> MQNEKLDHESVTQAMQPKDTPELRALYKSFEEESIIPLWTQLGDLMPIHPKSKAVPHVWKWSTLLRLARKSGELVPVGRGGERRALGLANPGLGGNAYISPTMWAAIQYLGPRETAPEHRHSQNAFRFVVEGEGVWTVVNGDPVRMSRGDLLLTPGWCFHGHMNDTDQPMAWIDGLDIPFSQQMDVGFFEFGSDRVTDYATPNFSRGERLWCHPGLRPLSGLQNTVASPIGAYRWEFTDRALTEQLLLEDEGQPATVAPGHAAIRYVNPTTGGDVMPTLRCEFHRLRAGTETATRNEVGSTVFQVFEGAGAVV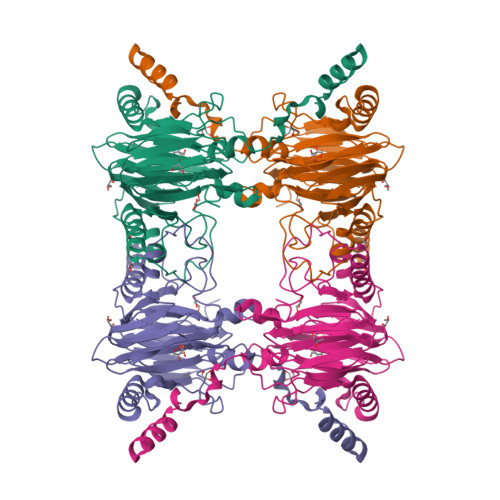MNGETTKLEKGDMFVVPSWVPWSLQAETQFDLFRFSDAPIMEALSFMRTKIEGQK> A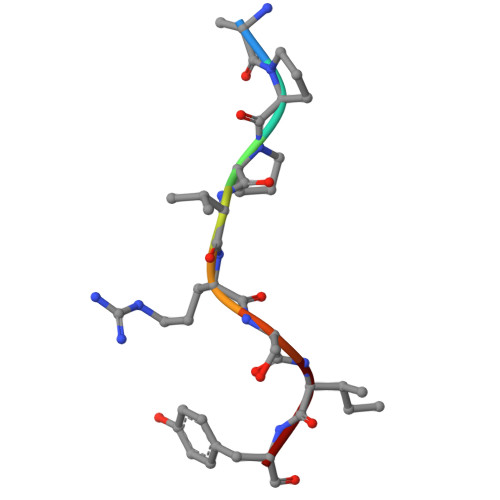PPVRSIY>GMEQATRTIYSEYAAYPETQGIIAVEKRQPRDSLTDQFDVLLLVITRDPSVEWTVKHYRLNTLRVSLHLVHEQVLSRWLILNANRRAVHWVSEGTIIFERNDYLTDLKKQLRNFPETERCLQMSLSFAKLLRRFQDGRNLFSRGNYYDAYTHVHHALHHLARLSVLEKGAHPEVVVWEQARLDDPDVYKLYEQLLLSEETLEQRIHLALIGLEHLLQSKVLSGGKYLFEVMRERDRPWTMHELMEESRLTELKVDLGSLVDFFIRK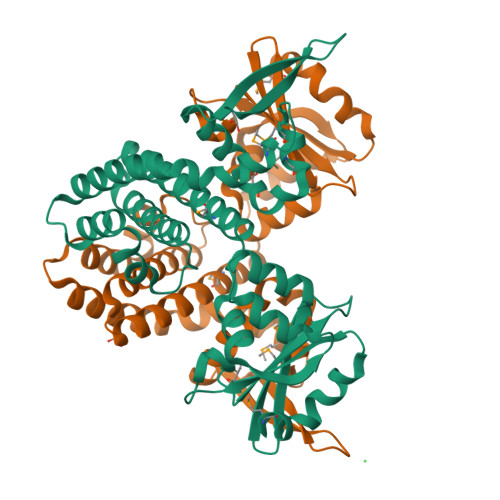GLIRISYQRTKGLGVELVTYEPVV[3x]> MAHHHHHHKLGERVSRTEMTDVTPAQLGETKVRVLNASGRGGQAADVAGALKDLGFTQPTAANDPVYADTRLDCQGQIRFGTAGQATAAAVW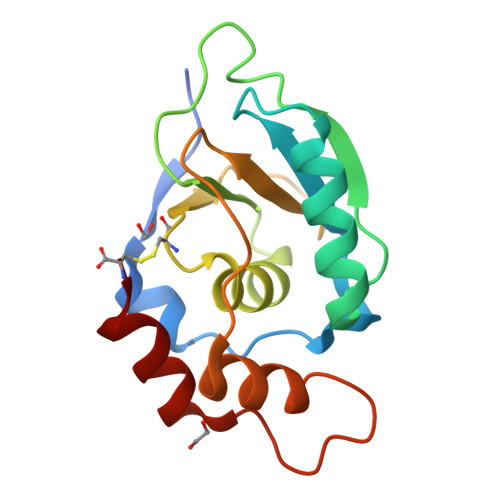LVAPCTELFNDGRADDSVDLVLGTDFTTLAHNDDIDAVLSSLRPGATQPPDPTLIAKIHASSC>[2x]SNAMATSEASRDESVQTVSTARGEVDCVIVGAGPPVLVVHGSPGGHDAGLAMARFLVAEGLRAIVVDRPGYFGTPLGSGVTPDEQAELYAALFDALGLAAAGVLCWSGGGPSSYRLAARHPDRVRALVSVAAVSHRYHFDGEKGAEKVLMG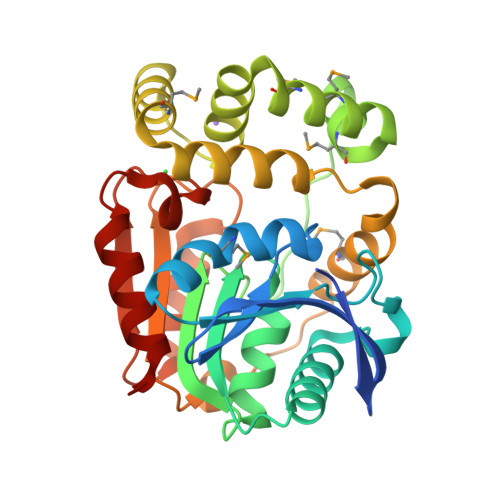TGLGRRMLQLMAAHTPEKLVSATIAAEGHLSKEHVAERVAQIMADPDKERFTLELAVSANHSGPRKAGFDNDMDQFARIDSLELDRITAPTLVVSGTADSDVDPEFSRFAAAQIAGSELVHLDAGTHLAFWVHPDSGPVRRRAAELLRAGG>AFAKISQVAHYVPEQVVTNHDLAQIMDTNDEWISSRTGIRQRHISRTESTSDLATEVAKKLMAKAGITGKELDFIILATITPDSMMPSTAARVQANIGANKAFAFDLTAACSGFVFALSTAEKFIASGRFQKGLVIGSETLSKAVDWSDRSTAVLFGDGAGGVLLEASEQEHFLAESLNSDGSRSECLTYGHSGLHSPFSDQESADSFLKMDGRTVFDFAIRDVAKSIKQTIDESPIEVTDLDYLLLHQANDRILDKMARKIGVDRAKLPANMMEYGNTSAASIPILLSECVEQGLI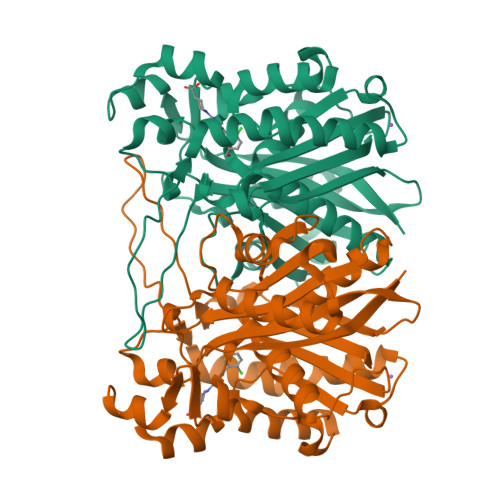PLDGSQTVLLSGFGGGLTWGTLILTI[2x]>MSREEVESLIQEVLEVYPEKARKDRNKHLAVNDPAVTQSKKCIISNKKSQPGLMTIRGCAYAGSKGVVWGPIKDMIHISHGPVGCGQYSRAGRRNYYIGTTGVNAFVTMNFTSDFQEKDIVFGGDKKLAKLIDEVETLFPLNKGISVQSECPIGLIGDDIESVSKVKGAELSKTIVPVRCEGFRGVSQSLGHHIANDAVRDWVLGKRDEDTTFASTPYDVAIIGDYNIGGDAWSSRILLEEMGLRCVAQWSGDGSISEIELTPKVKLNLVHCYRSMNYISRHMEEKYGIPWMEYNFFGPTKTIESLRAIAAKFDESIQKKCEEVIAKYKPEWEAVVAKYRPRLEGKRVMLYIGGLRPRHVIGAYEDLGMEVVGTGYEFAHNDDYDRTMKEMGDSTLLYDDVTGYEFEEFVKRIKPDLIGSGIKEKFIFQKMGIPFREMHSWDYSGPYHGFDGFAIFARDMDMTLNNPCWKKLQAPWE[2x];>[2x]SQQVDKIKASYPLFLDQDYKDMLAKKRDGFEEKYPQDKIDEVFQWTTTKEYQELNFQREALTVNPAKACQPLGAVLCALGFEKTMPYVHGSQGCVAYFRSYFNRHFREPVSCVSDSMTEDAAVFGGQQNMKDGLQNCKATYKPDMIAVSTTCMAEVIGDDLNAFINNSKKEGFIPDEFPVPFAHTPSFVGSHVTGWDNMFEGIARYFTLKSMDDKVVGSNKKINIVPGFETYLGNFRVIKRMLSEMGVGYSLLSDPEEVLDTPADGQFRMYAGGTTQEEMKDAPNALNTVLLQPWHLEKTKKFVEGTWKHEVPKLNIPMGLDWTDEFLMKVSEISGQPIPASLTKERGRLVDMMTDSHTWLHGKRFALWGDPDFVMGLVKFLLELGCEPVHILCHNGNKRWKKAVDAILAASPYGKNATVYIGKDLWHLRSLVFTDKPDFMIGNSYGKFIQRDTLHKGKEFEVPLIRIGFPIFDRHHLHRSTTLGYEGAMQILTTLVNSILERLDEETRGMQATDYNHDLVR

Nitrogenase catalyzes the ATP-dependent reduction of dinitrogen to ammonia during the process of biological nitrogen fixation that is essential for sustaining life. The Fe-protein mediates ATP-dependent electron transfer (ET) through its [4Fe:4S] cluster to the intermediate [8Fe:7S] P-cluster in the MoFe-protein; the electrons are subsequently shuttled to a [7Fe:1Mo:9S:1C]-R-homocitrate metallocluster, the FeMo-cofactor, within the active site of the MoFe-protein. The active site FeMo-cofactor contains a [7Fe:1Mo:9S:1C] metallocluster coordinated with an R-homocitrate (HCA) molecule.

To determine whether the features of the MoFeAlkaline-inactivated state stem solely from the loss of HCA, we characterized the homocitrate-deficient MoFe-protein purified from the homocitrate synthase (nifV) deletion strain of A. vinelandii (MoFeΔNifV). Like MoFeAlkaline-inactivated, MoFeΔNifV showed similar SEC shifts in elution time relative to MoFeAs-isolated and had diminished levels of acetylene reduction. Likewise, EPR spectroscopy revealed a loss of the canonical as-isolated S = 3/2 signal from the FeMo-cofactor in the MoFeΔNifV form, comparable to the MoFeAlkaline-inactivated state. The single particle cryoEM structure of MoFeΔNifV also showed asymmetric disordering of residues 14–19, 25–26, and 408–417 in one of the α-subunits. No density was observed at the canonical HCA position within the active site of the disordered α-subunit, but a smaller density remains in the HCA pocket within the corresponding ordered α-subunit. No homocitrate was detected by IC-MS, but citrate was isolated from the MoFeΔNifV sample at a molar ratio of 0.2-mole citrate per mole MoFeΔNifV. In our work, ~39 moles Fe and 1.8 Mo per molecule of MoFeΔNifV were detected by ICP-MS of the purified protein, suggestive of a full complement of clusters. The Phe α300 side chain is flipped in the disordered α-subunit of MoFeΔNifV, however, His α362, His α442, and His α451 remain close to their resting state positions in both dimers, preventing the formation of the histidine coordination site. In addition, while Gln β93 remained close to the as-isolated position in MoFeΔNifV, Trp α253 was observed to undergo the same conformational change as observed in the MoFeAlkaline-inactivated state in its more ordered α-subunit.>MRGSHHHHHHGSSLTTAAPLLALLRENQDSVKTYALESINNVVDQLWSEISNELPDIEALYDDDTFSDREMAALIASKVYYNLGEYESAVKYALAAKDRFDIDEKSQFVETIVSKSIEMYVQEASKQYTKDEQFYTKDIIDPKLTSIFERMIEKCLKASELKLALGIALEGYRLDIIESALKSKLDQDSTSENVKIINYLLTLAITTVTNSKFRSSILRKSFDFLMNMPNCDYLTLNKVVVNLNDAGLALQLFKKLKEENDEGLSAQIAFDLVSSASQQLLEILVTELTAQGYDPALLNILSGLPTCDYYNTFLLNNKNIDIGLLNKSKSSLDGKFSLFHTAVSVANGFMHAGTTDNSFIKANLPWLGKAQNWAKFTATASLGVIHKGNLLEGKKVMAPYLPGSRASSRFIKGGSLYGLGLIYAGFGRDTTDYLKNIIVENSGTSGDEDVDVLLHGASLGIGLAAMGSANIEVYEALKEVLYNDSATSGEAAALGMGLCMLGTGKPEAIHDMFTYSQETQHGNITRGLAVGLALINYGRQELADDLITKMLASDESLLRYGGAFTIALAYAGTGNNSAVKRLLHVAVSDSNDDVRRAAVIALGFVLLRDYTTVPRIVQLLSKSHNAHVRCGTAFALGIACAGKGLQSAIDVLDPLTKDPVDFVRQAAMIALSMILIQQTEKLNPQVADINKNFLSVITNKHQEGLAKFGACVAQGIMNAGGRNVTIQ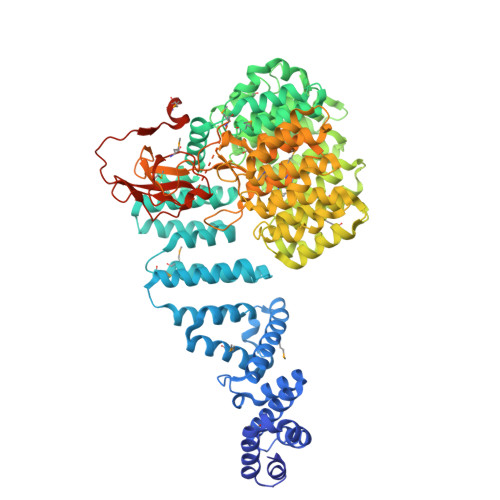LENADTGTLDTKSVVGLVMFSQFWYWFPLAHFLSLSFTPTTVIGIRGSDQAIPKFQMNCYAKEDAFSYPRMYEEASGKEVEKVATAVLSTTARAKARAKKTKKEKGPNEEEKKKEHEEKEKERETNKKGIKETKENDEEFYKNKYSSKPYKVDNMTRILPQQSRYISFIKDDRFVPVRKFKGNNGVVVLRDREPKEPVALIETVRQMKDVNAPLPTPFKVDDNVDFPSALQPSLIS[2x]> MDAELKIFVSSQHQPDIWRKALDQYEAKTPGVKVVIETGGNTSEMQAQYLNTVMSAKDSSLDVLMLDVIRPAQFATAGWTSDFSGKDLSAYLPTYAEANTVNGKIVALPAFADSMFLYYRKDL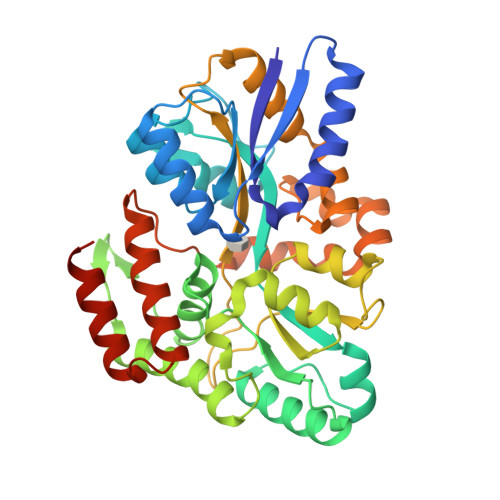LDKYGIKPPTTWDELKEASKKVMEGEKNPELQGLSFQGKAIEGAVCTFLLPYWSEGKSLVENGKLNFDNKAAVDSLKLWKSFVDDGISKKNISEVATDDTRKEFQAGKVLFAVNWSYAWTHFQGKESQVNDKVGVARLPAVKGGEQTTCLGGWEFGVSAYSKQQDEAKKLVEYLSSQDVSKFMAINAALLPTYAALYKDADVTKTIPWFADALPVVETAKARPVTPRYNEVSETIRTTVNGVLAGVMTPEDGAKQMESRLRRVLRLEHHHHHH> SPQPLEQIKLSESQLSGRVGMIEMDLASGRTLTAWRADERFPMMSTFKVVLCGAVLARVDAGDEQLERKIHYRQQDLVDYSPVSEKHLADGMTVGELCAAAITMSDNSAANLLLATVGGPAGLTAFLRQIGDNVTRLDRWETELNEALPGDARDTTTPASMAATLRKLLTSQRLSARSQRQLLQWMVDDRVAGPLIRSVLPAGWFIADRTGAGERGARGIVALLGPNNKAERIVVIYLRDTPASMAERNQQIAGIGAALIEHWQR

Bacteria harboring β-lactamase enzymes [E.C. 3.5.2.6] pose a significant threat to public health. These enzymes prevent β-lactam antibiotics from reaching their intended target, the penicillin binding proteins (PBPs). Sulbactam, tazobactam and clavulanic acid are mechanism-based inactivators as they share similarities with the β-lactam structure, the normal substrate for β-lactamases. Similar to a substrate, these inhibitors can, after acylation at catalytic residue S70, undergo several inhibitory reaction pathways including fragmentation in the active site and covalently cross-linking at S130.

In 2008, the K234R mutation was first identified in a clinical isolate harboring the SHV enzyme (SHV-56) which was found to be an IR β-lactamase and subsequently observed in two additional IR variants: SHV-72 and SHV-84. Previously, we determined the structure of the 1.08 Å IR apo K234R SHV variant. The presence of the larger guanidinium group of arginine in K234R SHV leads to two alternate conformations of this group which likely affected the nearby S130 position, which was also found to have two conformations. Most importantly, the C2 carboxylate participated in hydrogen bonding with R244, R234, T235 and both S130 conformations. There is however a minor shift observed in the C2 carboxyl moiety; this moiety has shifted 0.65Å away from the K234R substitution site, likely as a consequence of needing to accommodate the larger guanidinium side chain of arginine at position 234. Although the C2 tail occupies roughly the same location in both the wt SHV-1 and K234R SHV structures, it appears as though the tail is slightly disordered in the active site of the latter structure as evidenced by its weaker density. The R234 residue also adopts two conformations, as in the apo K234R SHV structure. In addition, we also observed two conformations for residue S130 with 35/65% occupancy. The residues with increased temperature factors are predominantly located in the Ω-loop which encompasses residues 164–179. Since residue K73 makes a salt-bridge interaction with E166 of the Ω-loop, it is possible that the K234R substitution can exert an effect on the Ω-loop via changes in position and dynamics of residues S130 and K73 which are both located between residue K234 and the Ω-loop residue E166.>[2x]MEFTTGLMSLDTALNEMLSRVTPLTAQETLPLVQCFGRILASDVVSPLDVPGFDNSAMDGYAVRLADIASGQPLPVAGKSFAGQPYHGEWPAGTCIR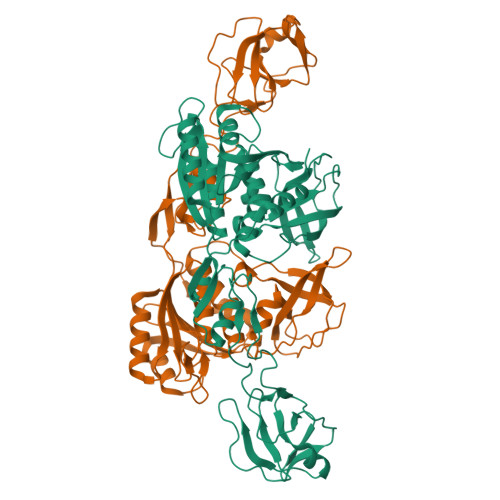IMTGAPVPEGCEAVVMQEQTEQMDNGVRFTAEVRSGQNIRRRGEDISAGAVVFPAGTRLTTAELPVIASLGIAEVPVIRKVRVALFSTGDELQLPGQPLGDGQIYDTNRLAVHLMLEQLGCEVINLGIIRDDPHALRAAFIEADSQADVVISSGGVSVGEADYTKTILEELGEIAFWKLAIQPGKPFAFGKLSNSWFCGLPGNPVSATLTFYQLVQPLLAKLSGNTASGLPARQRVRTASRLKKTPGRLDFQRGVLQRNADGELEVTTTGHQGSHIFSSFSLGNCFIVLERDRGNVEVGEWVEVEPFNALFGGL>[4x]SNAMDSRFLPATAFIDPEGRNRNEVERLVQQVVDLILAKLTGAAERPPMPETVDLPGPITIPEAAATEATLLQAIRDMVDGSMNPANPGYIGHMDPMPATMAILGDLVAAAVNNNMLSLEMSPSFSRLETLLLRAIAGLFGLGEQAGGVLTSGGSLANLQALAVARNVAFDSVEPGITGLAQRPVIFASEAAHTSLQKAAMLLGLGTAAVIPVRATAD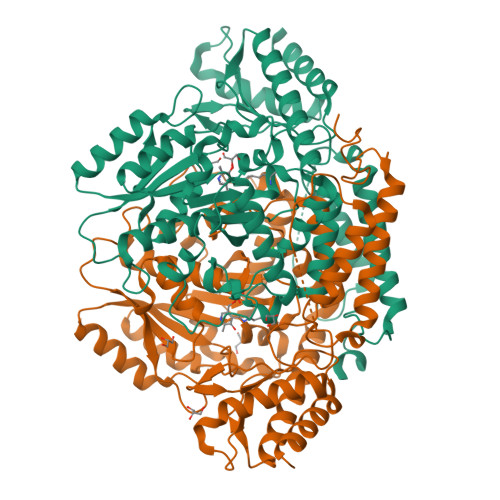SRMDPEDLRARIDQARGAGQHPFCVVATAGTTTTGNIDPLAEIGAIAREHGLWFHVDAAYGGALVFSERHRWRLAGIEQADSITFNPQKWLYVAKTCAMVLFRDAGVLERAFRIPAPQMRATDGFINLGEIGVQGTRHADVVKLWLTLQHIGQQGYARLIDDGYRLAERVVEGVRQRPFLRLAGEIDTNIVCFRGEPDWLPAERWDDWNAALQALLLREGKIFLSLPVYRGGRWLRAVLLNPYTTDAVIDAMFKQIDRFAGRERGQER>ASGSMQGDPDVLRLLNEQLTSELTAINQYFLHSKMQDNWGFTELAAHTRAESFDEMRHAEEITDRILLLDGLPNYQRIGSLRIGQTLREQFEADLAIEYDVLNRLKPGIVMCREKQDTTSAVLL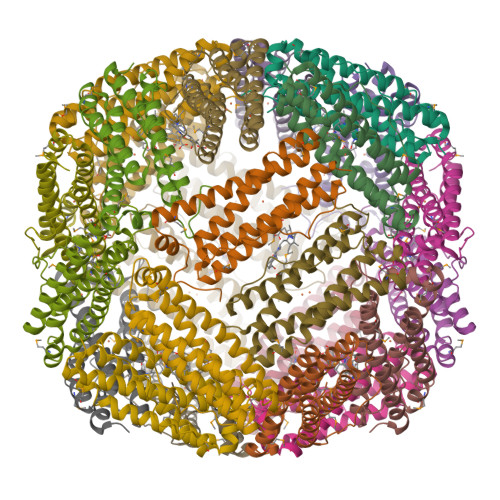EKIVADEEEHIDYLETQLELMDKLGEELYSAQCVSRPPTSAWSHPQFEK[6x]> MFRAAAPGQLRRAASLLRFQSTLVIAEHANDSLAPITLNTITAATRLGGEVSCLVAGTKCDKVAQDLCKVAGIAKVLVAQHDVYKGLLPEELTPLILATQKQFNYTHICAGASAFGKNLLPRVAAKLEVAPISDIIAIKSPDTFVRTIYAGNALCTVKCDEKVKVFSVRGTSFDAAATSGGSASSEKASSTSPVEISEWLDQKLTKSDRPELTGAKVVVSGGRGLKSGENFKLLYDLADQLHAAVGASRAAVDAGFVPNDMQVGQTGKIVAPELYIAVGISGAIQHLAGMKDSKTIVA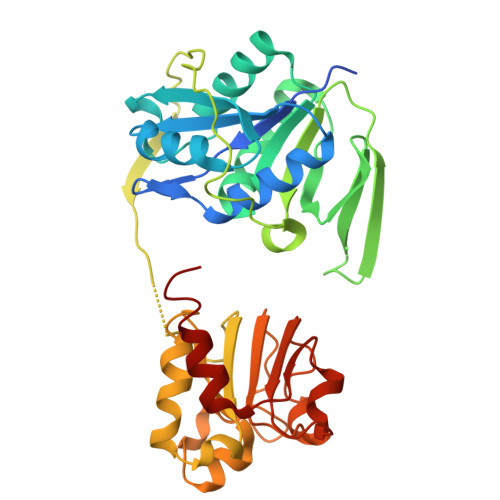INKDPEAPIFQVADYGIVADLFKVVPEMTEILKKK>[6x]ILGGREAEAHARPYMASVQ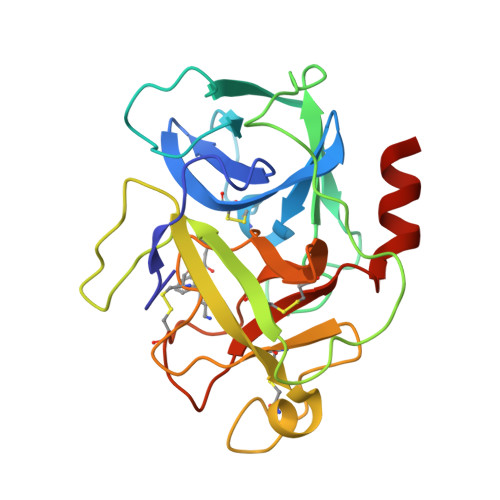LNGAHLCGGVLVAEQWVLSAAHCLEDAADGKVQVLLGAHSLSQPEPSKRLYDVLRAVPHPDSQPDTIDHDLLLLQLSEKATLGPAVRPLPWQRVDRDVAPGTLCDVAGWGIVNHAGRRPDSLQHVLLPVLDRATCNRRTHHDGAITERLMCAESNRRDSCKGDSGGPLVCGGVLEGVVTSGSRVCGNRKKPGIYTRVASYAAWIDSVLASAAA N-[4-(benzyloxy)phenyl]glycinamide | C15 H16 N2 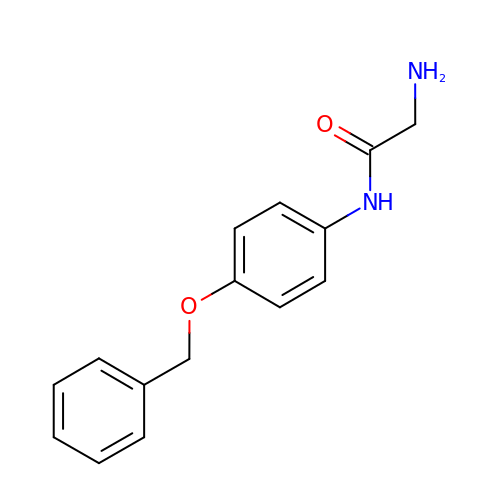O2 | YJPUATSIKWOSST-UHFFFAOYSA-N>[4x]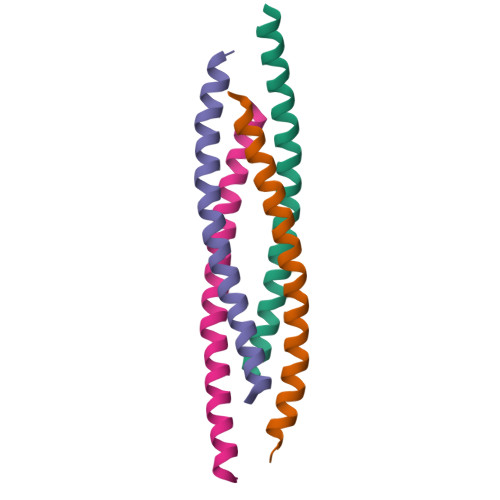MDMTQQEIFDKQRRLQELSEKVRTCHQEISALRKALQEKEAEVLQVLEDIQTI> ARTKQT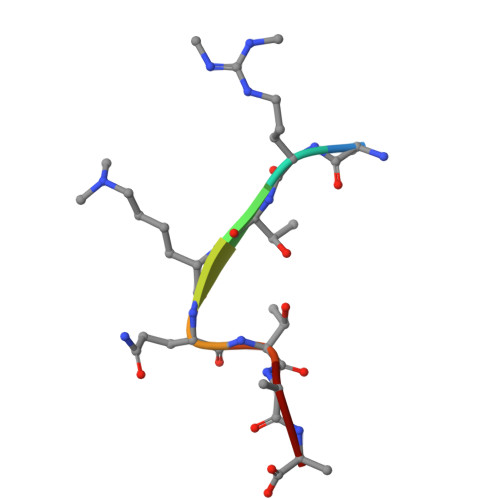AA~{N}-(2-chloranyl-6-methyl-phenyl)-2-[[3-(piperidin-4-ylcarbamoyl)-5-(trifluoromethyl)phenyl]amino]-1,3-thiazole-5-carboxamide 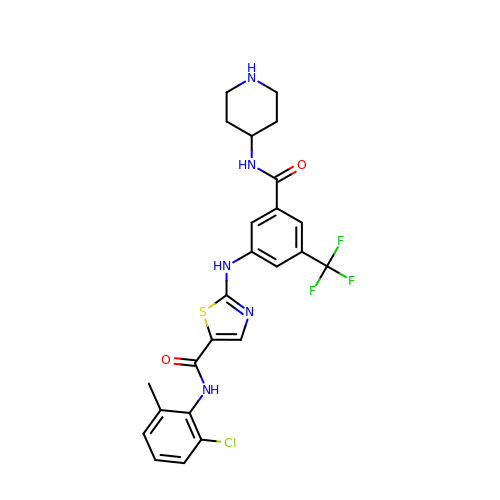| C24 H23 Cl F3 N5 O2 S | AMLFZMSYVMSKCA-UHFFFAOYSA-N> SHMSLTPDQIVAALQERGWQAEIVTEFS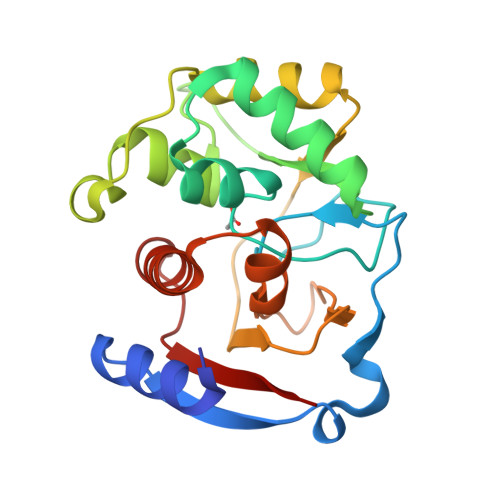LLNEMVDVDPQGILKCVDGRGSDNTQFCGPKMPGGIYAIAHNRGVTTLEGLKQITKEVASKGHVPSVHGDHSSDMLGCGFFKLWVTGRFDDMGYPRPQFDADQGAKAVENAGGVIEMHHGSHAEKVVYINLVENKTLEPDEDDQRFIVDGWAAGKFGLDVPKFLIAAAATVEMLGGPKKAKIVIP2-heptyl-3-iodanyl-1-oxidanyl-quinolin-4-one | C16 H20 I 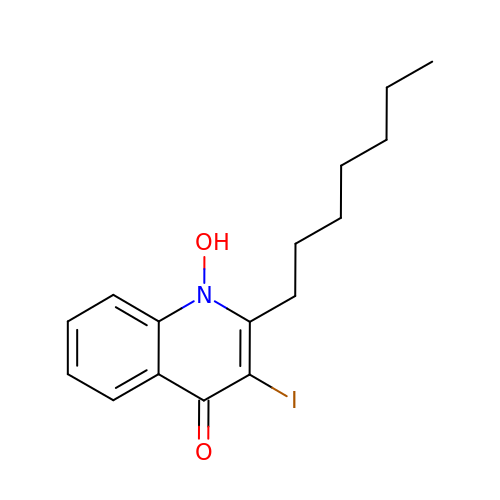N O2 | KWUZRGREQVAAQR-UHFFFAOYSA-N> NDTVLIAGAGHAGFQVAVSLRQAKYPGRIALINDEKHLPYQRPPLSKAYLKSGGDPNSLMFRPEKFFQDQAIELISDRMVSIDREGRKLLLASGTAIEYGHLVLATGARNRMLDVPNASLPDVLYLRTLDESEVLRQRMPDKKHVVVIGAGFIGLEFAATARAKGLEVDVVELAPRVMARVVTPEISSYFHDRHSGAGIRM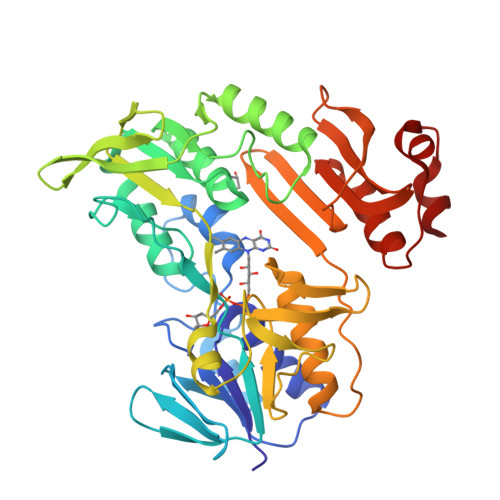HYGVRATEIAAEGDRVTGVVLSDGNTLPCDLVVVGVGVIPNVEIAAAAGLPTAAGIIVDQQLLTSDPHISAIGDCALFESVRFGETMRVESVQNATDQARCVAARLTGDAKPYDGYPWFWSDQGDDKLQIVGLTAGFDQVVIRGSVAERSFSAFCYKAGKLIGIESVNRAADHVFGRKILPLDKSVTPEQAADLSFDLKKAAA>MKLSPREVEKLGLHNAGYLAQKRLARGVRLNYTEAVALIASQIMEYARDGEKTVAQLMCLGQHLLGRRQVLPAVPHLLNAVQVEATFPDGTKLVTVHDPISRENGELQEALFGSLLPVPSLDKFAETKEDNRIPGEILCEDECLTLNIGRKAVILKVTSKGDRPIQVGSHYHFIEVNPYLTFDRRKAYGMRLNIAAGTAVRFEPGDCKSVTLVSIEGNKVIRGGNAIADGPVNETNLEAAMHAVRSKGFGHEEEKDASEGFTKEDPNCPFNTFIHRKEYANKYGPTTGDKIRLGDTNLLAEIEKDYALYGDECVFGGGKVIRDGMGQSCGHPPAISLDTVITNAVIIDYTGIIKADIGIKDGLIASIGKAGNPDIMNGVFSNMIIGANTEVIAGEGLIVTAGAIDCHVHYICPQLVYEAISSGITTLVGGGTGPAAGTRATTCTPSPTQMRLMLQSTDDLPLNFGFTGKGSSSKPDELHEIIKAGAMGLKLHEDWGSTPAAIDNCLTIAEHHDIQINIHTDTLNEAGFVEHSIAAFKGRTIHTYHSEGAGGGHAPDIIKVCGIKNVLPSSTNPTRPLTSNTIDEHLDMLMVCHHLDREIPEDLAFAHSRIRKKTIAAEDVLNDIGAISIISSDSQAMGRVGEVISRTWQTADKMKAQTGPLKCDSSDNDNFRIRRYIAKYTINPAIA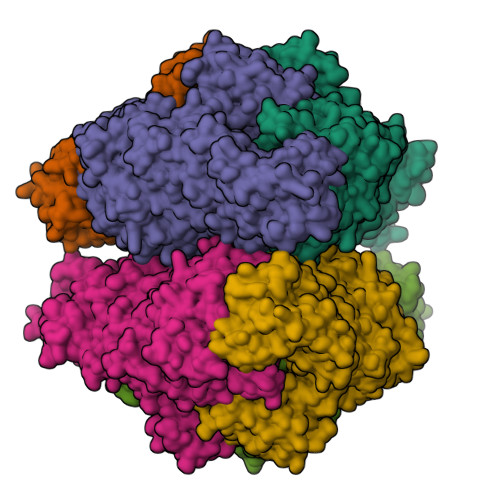NGFSQYVGSVEVGKLADLVMWKPSFFGTKPEMVIKGGMVAWADIGDPNASIPTPEPVKMRPMYGTLGKAGGALSIAFVSKAALDQRVNVLYGLNKRVEAVSNVRKLTKLDMKLNDALPEITVDPESYTVKADGKLLCVSEATTVPLSRNYFLF[6x]>MNIIKANVAAPDARVAITIAR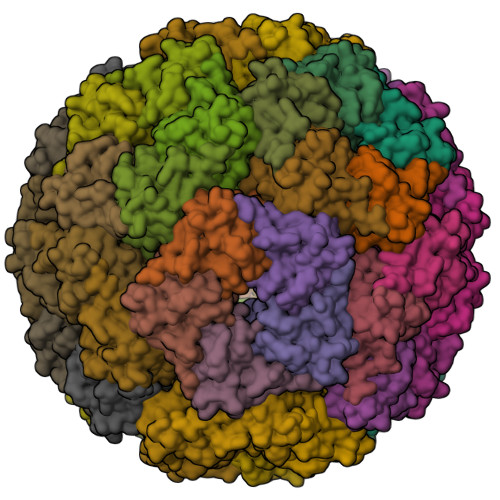FNQFINDSLLDGAVDALTRIGQVKDDNITVVWVPGAYELPLATEALAKSGKYDAVVALGTVIRGGTAHFEYVAGGASNGLASVAQDSGVPVAFGVLTTESIEQAIERAGTKAGNKGAEAALTALEMINVLKAIKA[30x]>[2x]MVMKLIGSHASPYTRKVRVVLAEKKIDYQFVLEDVWNADTQIHQFNPLGKVPCLVMDDGGALFDSRVIAEYADTLSPVARLIPPSGRERVEVRCWEALADGLLDAAV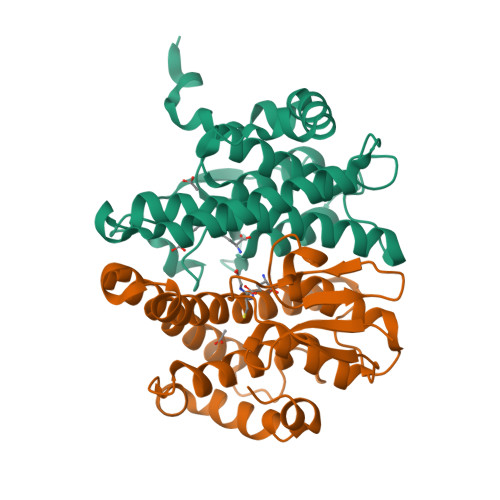ALRVEQTQRTPEQRSESWITRQHHKIDEALKAMSRGLADRTWCNGNHLTLADIAVGCALAYLDFRQPQVDWREQHANLAAFYTRIEKRPSFLETQPQAENLYFQSHHHHHHWSHPQFEK>HMKHSDEYKIRRERNNIAVRKSRDKAKMRNLETQHKVLELTAENERLQKKVEQLSRELSTLRNLFKQLPEPLLASSG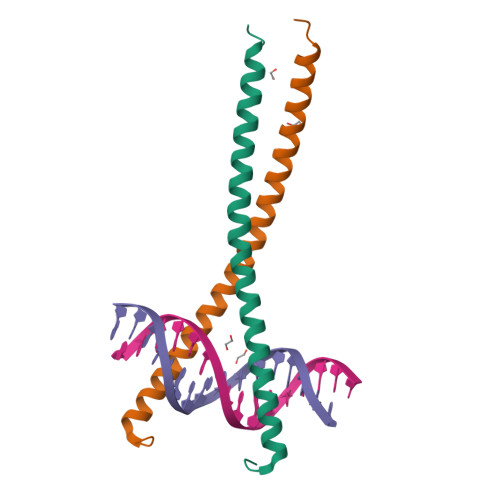H[2x]> IFGIDDLIFGLLFVGFVAGGVAGGYFWGRSNGGGGGASVSS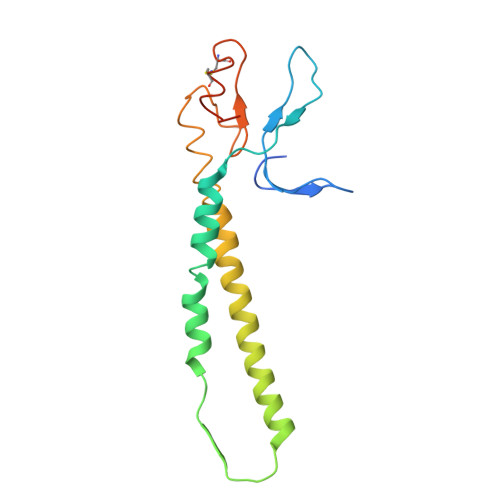TQAGFDKIGKDIQQLRNDTNAAIEGFNGRIAHDEQAIKNLAKEIEDARAEALVGELGIIRSLIVANISMNLKESLYELANQITKRGGGIAQEAGPGCWYVDSENCDASCKEYIFNFNGSATVPTL> MQALRRGAAIPSRLLPRRDSWMSLAPFVAPNNAAAWRKLRDGAQEVQTVIERQSTPGKPQQIDWAKWESQIAHKDILNCLKTFYTNQVQILDRALGALETAKTPAPCEGAEKGWALFDAALSACAKSVEKSEELLSNGARALWVSCSNPPVWKVNTNEWLDSDQYWQAFVEKHHFYSQYQPGVVDPEAPQEVEAFKQAWHSRMGKFNDRSDTPMLYAYMNELPSWEYYDLHRSAFLEHMTYFLVRTGGDFRFFPEMPPWQWLAHMENLRFKLLSVAQSRRSQLQLANLERERALDFLPVDVEHHGEEYTQKFLQYETELFQACAARLMGHFMFLCDPFIPVQSAEALSAVTRVDNGKGKLFSLGDDVNALFYLPEQQRRDVERPTQAVQTLLGHLEATGRPFNPCYSELLHVHAEVLEERGEHWLTAPGECVSQAFLRRLRTDDPAYEVYCSYFKEMYERFAGAKEVSMEDGRKRLATIEKNAQEEAAAYGLALKTMGSAELAHKAREGAAKLEQLRKAQEKAAGKSAQTVQENKM;> MNFSSSARWLAVRQSQTLGHTTRATVAAGRRVLAHSPAATEFTSFQSLHIGGDVCKLPLAVALGAAPSALGYGSAKHNQQRQYATLGSGWSFSKVQYTKYRITKPWTTDTTFDDIILSQPSKEDFAKFTKEAPLFLRFLKLVTDVEGRQEAFIQFAKRCENGLTVEKDVYVTKKELVDCLWKNGYTDTEINAFEIAFPADYKFHYPELAVLFDLTEEDCYKYCIRQRAATPEELVELKYTKPKNLVSSYGLCFLGVWFGLSNTVLSNAWFYSKTFPFGAVFYMLGSYFYRDIREKLWKEEKSLIHTAQENKNMGEESVYKQMKKYATDTKCLDYLSTFRTEVEDQIANYKVALVSQMRRQLTERLVEKLNGIQQAEKLIQGSLQDVMIREIVSSFKDLYKSRPELHDAAMQSAIQGLSGSDGAMDPVGAHFKASLQELAKVNLSTATADPMGTVVQRVAAVFQKREKEFLDTFTVKATEAQEIKTIVDKCHKGNTFDFHALSDEELRRLEQLYSTVNNRVGFETIHENSIKPVAPLSENSKGFVEFVNTQLEITKAKLRNARLTAFAHAFV;> MTIHSCLARRAVSVAASGARAFASGLGARAVAVGALQSARLLHTSSLRAAGAKISPSEMSRLLEERIAGWKTQTSTEEVGRVVSVGDGIARLFGLEGVQAGELVEFQNGMTGMALNLETDNVGVVIFGDDRSVLEGDSVKRTGRIVDVPIGPGLLGRVVDALGNPIDGKGPIPAKERRRVELKAPGIIPRKSVHEPMMTGLKCVDALVPVGRGQRELIIGDRQTGKTAVAVDAIINQKEINDSTDDESKKLYCIYVAVGQKRSTVAQIVKALEQRDAMKYTTVVAATASEAAPLQFLAPYSGCAMGEWFRDSGRHCVIIYDDLSKQATAYRQMSLLLRRPPGREAYPGDVFYLHSRLLERAAKMGDKSGGGSLTALPVIETQAGDVSAYIPTNVISITDGQIFLETELFYKGIRPAINVGLSVSRVGSAAQVKAMKQVAGTMKLELAQYREVAAFAQFGSDLDASTRQLLTRGTALTELLKQRQYSPMKNSVQVCVLYCGVKGYLDPLDPKEISRFESLFIDYINANHQDILKTIETEKELSEKTEAKLRAAVDEFVAMNEFKKK;> MALPLLASRRLFSSFVFRGQPSTLSSNLSLVRIRGLHGGSLSPPSATLPRAVQLFSSRIAFSTAAAEDSGASQTLEGRYASALFRVAKKKNQLEKVYGDLESVRNALKDSSEFRLFVDSPAVSVQQKLDVLRQLVNRYKFDPLTGNLLTTLVENKRLPMLARVADAFDAMYRKEKGEVKCLVTSAKPLSAQQQKEIVAALQNRAGTQARLIIDYAVSPQIMGGLVVRLGEQVLDFSVATRLDRLQSQLLAPL;> MLNFIPKRCPSVSLLFGKRPVQRIEVGQARHQLEIPVETIEKIYEGVDSRLEYHNKDYNAMKWKDFMKLKLDAYHLLEASQSETAAKSALSDLNWFSDLADIYSGQQTMAEMDVALKAQGEQKLSYPIQGKNIK

F-type ATP synthases are energy-converting membrane protein complexes that synthesize adenosine triphosphate (ATP) from ADP and inorganic phosphate. These universal enzymes function by using the energy stored in an electrochemical potential across the bioenergetic membrane by rotary catalysis. In mitochondria, F1Fo ATP synthase resides in the crista membrane where it is known to form dimers, which can further assemble into rows critical for inducing the membrane curvature and maintaining membrane potential and morphology. Here, we investigate the mechanism for the generation of the unique cristae in the Apicomplexa, using a combination of single-particle cryo-EM, cryo-ET and subtomogram averaging.

The peripheral stalk extends from the membrane-embedded part of Fo and attaches to the tip of F1, holding it stationary against the torque of the central stalk. In T. gondii the peripheral stalk is composed of subunit-b, d, ATPTG12 and OSCP. The attachment to F1 is mediated through OSCP, which adopts a fold conserved in prokaryotic and eukaryotic homologs. Subunit-b displays structural similarity with its bacterial, algal and mammalian counterparts, engaging in conserved interactions with the C-terminal domain of OSCP as observed in other structures. Compared to the yeast and mammalian ATP synthases, T. gondii displays an augmented peripheral stalk structure with extensions in subunit-b, subunit-d and the additional ATPTG12. Instead, the apicomplexan-conserved subunit ATPTG12 forms extensive interactions with subunit-b and d throughout the peripheral stalk structure. Interestingly, peripheral stalk subunit F6 (subunit h in yeast) is not found in T. gondii ATP synthase. Instead, the C-terminal extension of subunit-b, adopts a fold that structurally resembles subunit F6/h and provides supporting interactions with the long subunit-b helix. Both, the yeast subunit-h (on non-fermentable carbon sources) and the augmented T. gondii subunit-b are essential, suggesting a critical role in peripheral stalk assembly.> MPSQSGMNPADLSGLSGKELARARRAALSKQGKAAVSNKTASVNRSTKQAASSI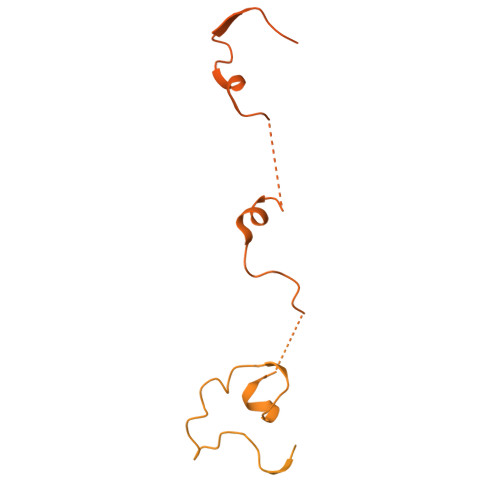NTNQVRSSVNEVPTDYQMADQLCSTIDHADFGTESNRVRDLCRQRREALSTIGKKAAKTTGKPSGRVRPQQSVVHNDAMIENAGDTNQSSSTSLNNELSEICSIADDMPERFGSQAKTVRDICRARRQALSERGTRAVPPKPQSQGGPGRNGYQIDGYLDTALHGRDAAKRHREMLCQYGRGTAPSCKPTGRVKNSVQSGNAAPKKVETGHTLSGGSVTGTQVDRKSHVTGNEPGTCRAVTGTEYVGTEQFTSFCNTSPKPNATKVNVTTTARGRPVSGTEVSRTEKVTGNESGVCRNVTGTEYMSNEAHFSLCGTAAKPSQADKVMFGATARTHQVVSGSDEFRPSSVTGNESGAKRTITGSQYADEGLARLTINGAPAKVARTHTFAGSDVTGTEIGRSTRVTGDESGSCRSISGTEYLSNEQFQSFCDTKPQRSPFKVGQDRTNKGQSVTGNLVDRSELVTGNEPGSCSRVTGSQYGQSKICGGGVGKVRSMRTLRGTSVSGQQLDHAPKMSGDERGGCMPVTGNEYYGREHFEPFCTSTPEPEAQSTEQSLTCEGQIISGTSVDASDLVTGNEIGEQQLISGDAYVGAQQTGCLPTSPRFNQTGNVQSMGFKNTNQPEQNFAPGEVMPTDFSIQTPARSAQNRITGNDIAPSGRITGPGMLATGLITGTPEFRHAARELVGSPQPMAMAMANRNKAAQAPVVQPEVVATQEKPELVCAPRSDQMDRVSGEGKERCHITGDDWSVNKHITGTAGQWASGRNPSMRGNARVVETSAFANRNVPKPEKPGSKITGSSGNDTQGSLITYSGGARG> GAMEDENILRNAVNLQVLKFHYPEIESIIDIASHVAVYQFDVGSQKWLKTSIEGTFFLVKDQRARVGYVILNRNSPENLYLFINHPSNVHLVDRYLIHRTENQHVVGLWMFDPND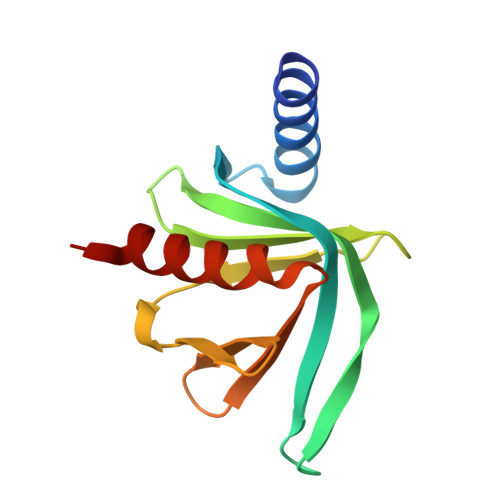MSRIFNIVKESLLR> MTLGTNQVSKTHSFMTVSLIELWERFGYYGMQALIVYFMVQRLGFDDSRANLVWSA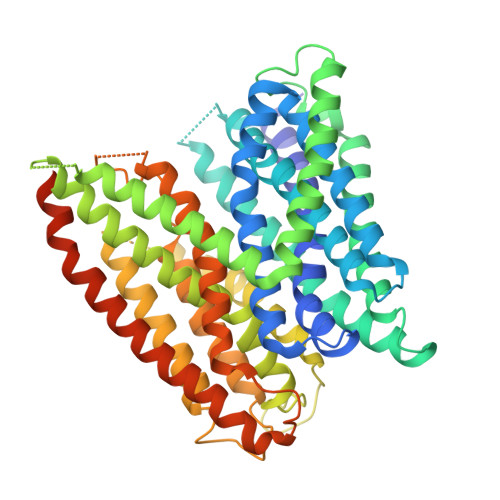CAALIYVSPAIGGWVGDKILGTKRTMLLGAGILSVGYALMTVPTENTWFMFSALGVIVVGNGLFKPNAGNLVRKIYEGDDSKIDSAFTIYYMAVNVGSTFSMLLTPWIKDYVNAQYGNEFGWHAAFAVCCVGILVGLGNYALMHKSLANYGSEPDTRPVNKKSLAIVLALAALSVVASAIILEYEDVARVFVYAAGVAVLGIFFHLIRTSEPSERAGLIAALILTVQTVFFFIFYQQMSTSLALFALRNVDWDFQVFGTHLWTWSPAQFQALNPIWIMVLSPVLAWSYSWAGRNNKDFSIAAKFALGFAVVAIGFFIYGFAGQFAVNGKTSSWVMIWGYASYSLGELLVSGLGLAMIARYVPARMGGFMMGAYFVASGISQYLGGVVANFASVPQDLVDPLQTLPVYTNLFNKLGVAAVVCTIIALAVLPLMRRLTESHHAHSSIENNAAASLRDVKAEQAENLYFQ Lipid transfer proteins (LTPs), also called non-specific lipid transfer proteins (nsLTPs), are known for their ability to bind and transport hydrophobic ligands. The biological role of nsLTPs is still not well understood. They transport these lipids between biological membranes primarily for defense, including structural adaptation, antimicrobial activity, and pathogenic resistance. We elucidated the crystal structures of Act c 10.0101 and Pun g 1.0101, nsLTP allergens from gold kiwifruit and pomegranate, respectively. These allergens both belong to the subfamily of 9-kDa LTPs.

Act c 10.0101 crystallized in the P21 space group with two protein molecules in the asymmetric units. The model was refined to 1.95Å resolution. The crystal structure corresponds to a closed apo form of the protein. Both protein chains include residues 1–92 (mature form of the protein) that are folded into a compact, mainly α-helical structure that is characteristic for nsLTPs. The protein chains adopt very similar conformations and they superposed with Root Mean Square Deviation (RMSD) value of 0.3Å over 92 Cα. The Act c 10.0101 structure is stabilized by four disulfide bridges that are formed by the following pairs of cysteine residues: Cys4–Cys51, Cys14–Cys28, Cys29–Cys74, and Cys49–Cys88. We have identified three additional amino acids at the C-terminal end of the protein and modeled these amino acids as Lys-Ile-Ser, which is consistent with the sequence that is observed in homologous Act d 10.0101 and Act d 10.0201, as well as in agreement with the results of mass spectrometric analysis of the sample used for crystallization. The crystal structure revealed that Lys90 is solvent exposed, the side chain of Ile91 points toward the hydrophobic core of the protein, and the C-terminal carboxyl group of Ser92 forms a salt bridge with Arg45. The covalent ligand binding was shown in the case of oxylipin-conjugated barley 9-kDa LTP, where Asp7 of this nsLTP is responsible for the formation of the bond between the protein and lipid. This aspartic acid residue is conserved in Act c 10.0101 (Asp8), Act d 10.0101, Act d 10.0201, chickpea Cic a 3, tomato Sola l 7.0101, and wheat Tri a 14.0201, which suggests that these nsLTPs may have a similar mode of ligand binding and may also bind oxylipins. The difference in likely modes of ligand binding for Act c 10.0101 is not only related to the presence of the conserved aspartic acid residue in kiwifruit protein, but also the absence of a tyrosine residue in the Ω loop.

>[2x]AVSCGQVDTSLTPCLTYLTKGGTPSTQCCSGVRSLKSMTGTKADRQAACNCLKQAAARYQGIKDAAAAALSQKCGVQLSVPISRKTDCSKIS> MSSIDNDSDVDLTEDLAVAKIVKENPVARKMVRYILSRGESQNSIITRNKLQSVIHEAAREEN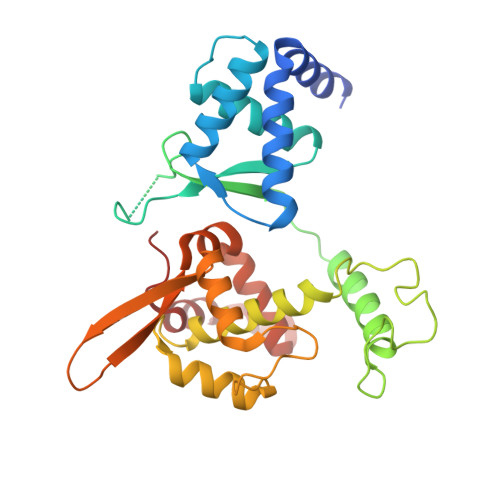IAKPSFSKMFMDINAILYNVYGFELQGLPSKNNMNAGGNGSNSNTNKSMPEPLGHRAQKFILLNNVPHSKNFDDFKILQSAHTYEELIVTGEYIGDDIASGTSNTLESKLSTDRDLVYKGVLSVILCIVFFSKNNILHQELIKFLETFGIPSDGSKIAILNITIEDLIKSLEKREYIVRLEEKSDTDGEVISYRIGRRTQAELGLESLEKLVQEIMGLEKEQTKSLHDDIIKSIGDSYSI>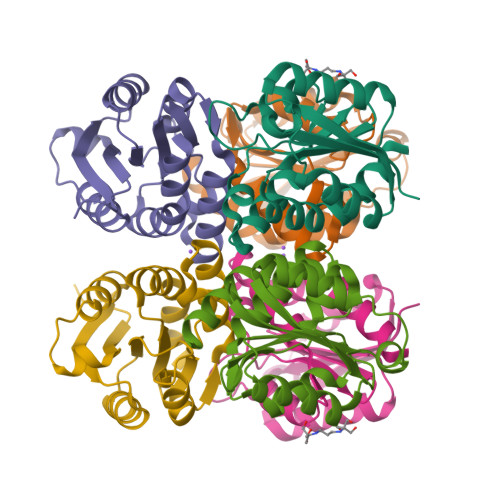[3x]GPGSMVNADAQLSDLGYSVAPMEQGAELVVGRALVVVVDDRTAHGDEDHSGPLVTELLTEAGFVVDGVVAVEADEVDIRNALNTAVIGGVDLVVSVGGTGVTPRDVTPESTREILDREILGIAEAIRASGLSAGIIDAGLSRGLAGVSGSTLVVNLAGSRYAVRDGMATLNPLAAHIIGQLSSLE>MHHHHHHMPIIEQVRAREILDSRGNPTVEVEVALIDGTFARAAVPSGASTGEHEAVELRDGGDRYGGKGVQKAVQAVLDEIGPAVIGLNADDQRLVDQALVDLDGTPDKSRLGGNAILGVSLAVAKAAADSAELPLFRYVGGPNAHILPVPMMNILNGGAHADTAVDIQEFMVAPIGAPSFVEALRWGAEVYHALKSVLKKEGLSTGLGDEGGFAPDVAGTTAALDLISRAIESAGLRPGADVALALDAAATEFFTDGTGYVFEGTTRTADQMTEFYAGLLGAYPLVSIEDPLSEDDWDGWAALTASIGDRVQIVGDDIFVTNPERLEEGIERGVANALLVKVNQIGTLTETLDAVTLAHHGGYRTMISHRSGETEDTMIADLAVAIGSGQIKTGAPARSERVAKYNQLLRIEEALGDAARYAGDLAF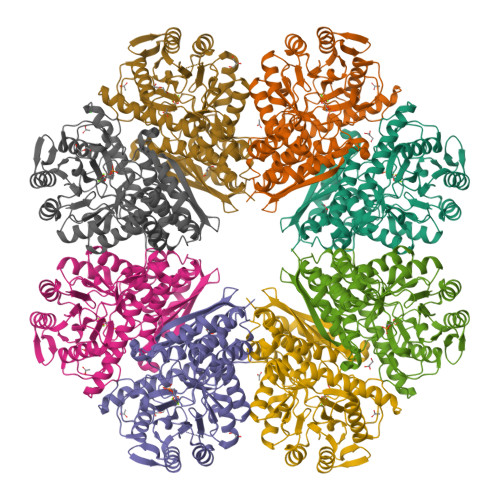PRFACETK[4x]> MKIRDLLKARRGPLFSFEFFPPKDPEGEEALFRTLEELKAFRPAFVSITYGAMGSTRERSVAWAQRIQSLGLNPLAHLTVAGQSRKEVAEVLHRFVESGVENLLALRGDPPRGERVFRPHPEGFRYAAELVALIRERYGDRVSVGGAAYPEGHPESESLEADLRHFKAKVEAGLDFAITQLFFNNAHYFGFLERARRAGIGIPILPGIMPVTSYRQLRRFTEVCGASIPGPLLAKLERHQDDPK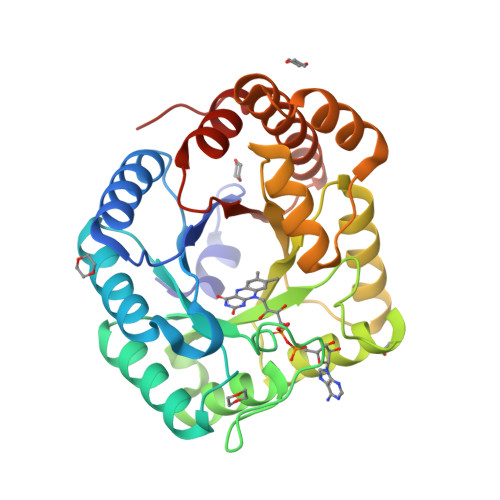AVLEIGVEHAVRQVAELLEAGVEGVHFYTLNKSPATRMVLERLGLRPASGQP> MTTTDKTDSRLGPYVEHLGLQFERIDPDRAVAYWSVRADLLQPHGILHGGVHCAVVESVASAAADRWLGDRGTVVGVSNSTDFFAPATVADGRLTSTALPVHRGATQQVWS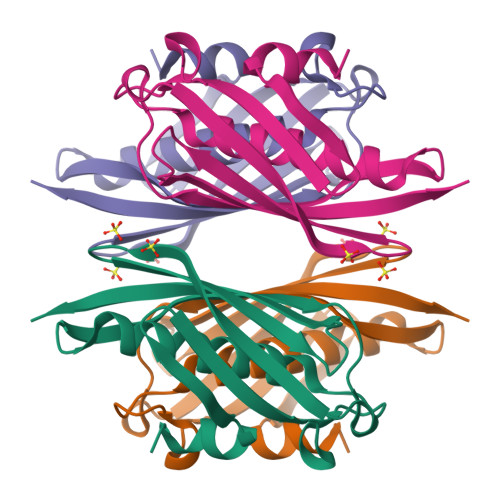VETVDAAGRLVARGQVRLHNLRLEHHHHHH Our model protein for comparing methods of RT structure determination is the coelomic hemoglobin from the marine annelid Amphitrite ornata. Named dehaloperoxidase (DHP; Chen et al., 1996; Zhang et al., 1996), this O2-transport protein is capable of oxidizing a wide array of substrates by either electron or O-atom transfer. DHP exhibits four activities common to heme proteins, peroxidase, peroxy­gen­ase, oxidase and oxygenase, with each activity employing an Fe(IV)-oxo (ferryl) intermediate. In this study, structures of a multifunctional globin, dehaloperoxidase B (DHP-B), obtained using several methods of room-temperature crystallographic structure determination are described and compared.

As well as this, we present an X-ray crystal structure that was determined from the same crystal as previously used for collection of the neutron data (data set NX-Xray). Following the completion of neutron data collection, RT X-ray diffraction data were collected from the same crystal using an in-house source (NX-Xray). The Fe distance to O-MPEG in the NX-Xray structure is 2.23 Å, which is much shorter than in the NX structure (3.04 Å). During RT data collection, we assume that the ferric heme centre of protomer A was rapidly photoreduced to the ferrous state due to the ionizing properties of the X-ray beam, which is consistent with extensive studies on heme proteins and specifically of DHP. This reduction could lead to displacement of the MPEG molecule as DHP forms the oxyferrous state. The SSX, SLX and NX-Xray structures incurred X-ray doses ranging from 21.8 to 83 kGy. While these are very low doses, small enough to avoid typical site-specific damage to bound ligands or proteins such as decarboxylation of side chains or reduction of disulfide bonds, we expect the photoreduction of the heme iron to occur after just a few kGy. For the SSX, SLX and NX-Xray structures site-specific radiation damage may also be a contributing factor.

>GFKQDIATLRGDLRTYAQDIFLAFLNKYPDEKRNFKNYVGKSDQELKSMAKFGDHTEKVFNLMMEVADRATDCVPLASDASTLVQMKQHSGLTTGNFEKLFVALVEYMRASGQSFDSQSWDRFGKNLVSALSSAGMK[2x]~{N}1-(3-chloranyl-[1,2,4]triazolo[4,3-b]pyridazin-6-yl)-~{N}4-[2-(trifluoromethyl)pyrimidin-4-yl]cyclohexane-1,4-diamine | C16 H16 Cl F3 N8 | 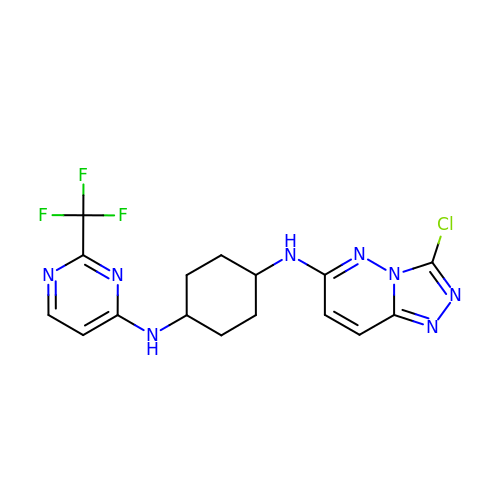ONWCUJRODWUZTD-AOOOYVTPSA-N(2Z,3R,4S,5R,6R)-2-[(4-aminobutyl)imino]-6-(hydroxymethyl)piperidine-3,4,5-triol | C10 H21 N3 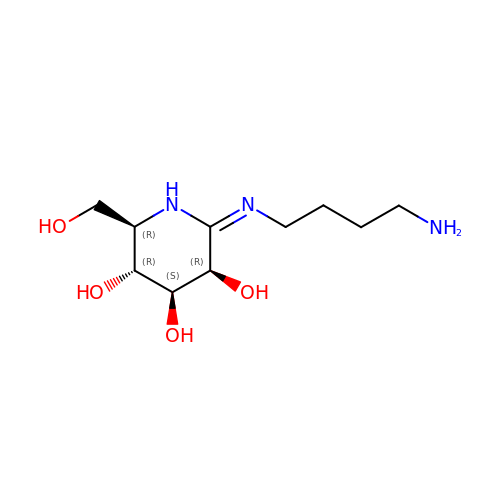O4 | ZLLQXILWWIGNJJ-HXFLIBJXSA-N>[2x]SSKPGPVQVVLVQKDQH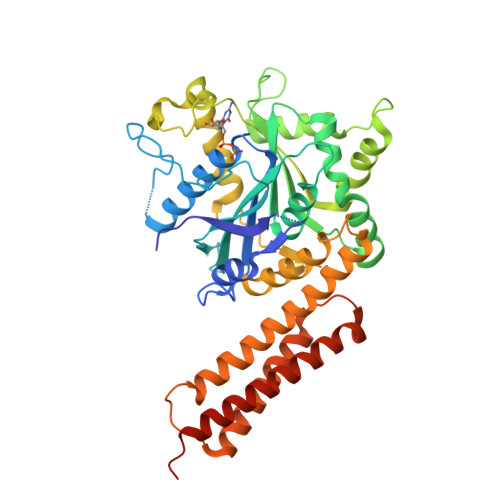SFELDEKALASILLQDHIRDLDVVVVSVAGAFRKGKSFILDFMLRYLYSQKESGHSNWLGDPEEPLTGFSWRGGSDPETTGIQIWSEVFTVEKPGGKKVAVVLMDTQGAFDSQSTVKDCATIFALSTMTSSVQIYNLSQNIQEDDLQQLQLFTEYGRLAMDEIFQKPFQTLMFLVRDWSFPYEYSYGLQGGMAFLDKRLQVKEHQHEEIQNVRNHIHSCFSDVTCFLLPHPGLQVATSPDFDGKLKDIAGEFKEQLQALIPYVLNPSKLMEKEINGSKVTCRGLLEYFKAYIKIYQGEDLPHPKSMLQATAEANNLAAAASAKDIYYNNMEEVCGGEKPYLSPDILEEKHCEFKQLALDHFKKTKKMGGKDFSFRYQQELEEEIKELYENFCKHNGSKNVFSTFRAALHHHHHH>[2x]MFPQDFLFGVAMSGFQFEMGKENSKDENTDWYIWTHDLQNQANGVVSRDLVEEG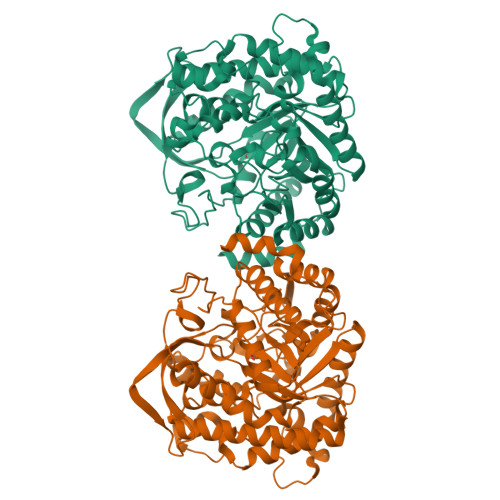ADYWNSYARVHELCSRIGMNVIRIGIEWSRIFPNPTHGIKDPSQIADMKVVEHYKQIIEDAKSRGLKVIVNLNHFTLPLWLHDPIRVSRFNDFSRSGWLDDRSVHEFTKFATFCAKSFDDVDAFTTMNEPNVVAKLGYFGRLSGFPPSLLNIDLYEKALDNQILAHNKAYETMKQFTNKPVGIIYATSWCEGDDARNDAMELENWYFLDRVIDRIDFLGVNYYTRAIVKRTPSVLSSSSGRIKINWSFVPGFGGSCQRNSKSLDGRPSTDNGWEIYPEGLGYVLRSCRDRYKKPLYVTENGVADDRDIYRPYSLLAHLKIVEDCLKENMDLRGYMHWSIIDNFEWPMGYSMRFGLVRVDFKQKLFTPRPSYYLFGQIINSRTTEPFLNLLKAWE(4aS)-5-[(2,4-diaminopteridin-6-yl)methyl]-4a,5-dihydro-2H-dibenzo[b,f]azepin-8-ol 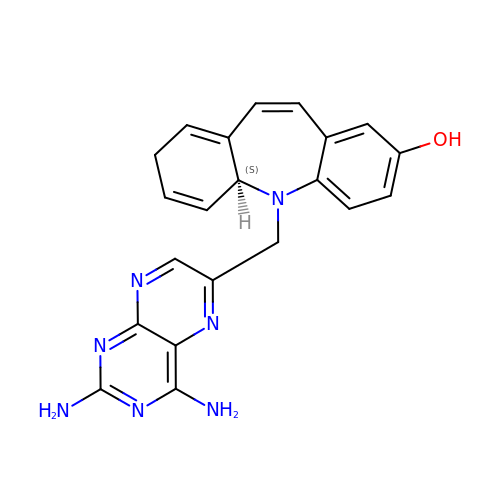| C21 H19 N7 O | PCBWLKUEKANDCL-INIZCTEOSA-N> MGEQRSVARMSKSAYRHPLAPKDPSQRNVTIPIRASRAAASASSSSASAALSAEDLKKQAQKVLLLQMQQKVLWEGTV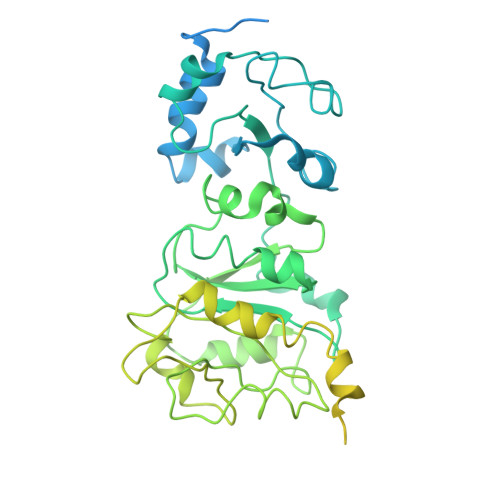IDDVNHALVQHFLKLSTNDKYRQARQMLVIGGRAMIEELCRAGHRPRHLMVECGKPIPEFLHDRRKTDVVLVDRSVSVAVTPGSDGYVGDFAIPTPPMKEKLIANHQRLNRVLVLDNIEDPGVLGTLLRTASGYQYDAIIATNHCADLYDHRVVRAARGAHFQTSVPIYTLKDEDGDDVYGLLNHIVERNNLLPLCYIAQADAAGVDGETAGTQTGFVSSPEAPVGRVFRSSVVGAAPVPLPAPRQSDSSYAASLSRELASVSQAREELLSDFCLDRFTGASSAEDDARSGYILFAGPNHKRNMLRRLERSLSRRSTRLLLDSLPSPSEAPSDLLIAMSVVLYTLRPRGNWDYLPVDTKHEHSTLDLQAKHASVDIGVNRLRVSVDDINLDEAEQQDRAHEANEFMRWRRLARRRGSDYDHWMAAEQRRVQAMVRRERQRRVAPWMPLRDAKTKPMPDWVPNIIDEYRQSLDRDALARERDISTSYQRPPR> RVQKEGVLRVITRNSPATYFQDRNGETGFEYELAKRFAERLGVELKIETADNLDDLY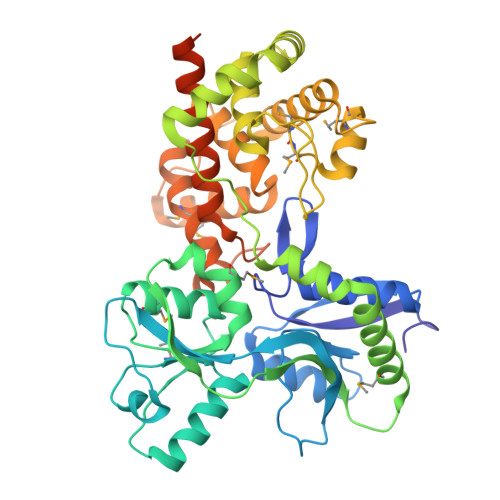AQLSREGGPALAAAGLTPGREDDASVRYSHTYLDVTPQIIYRNGQQRPTRPEDLVGKRIMVLKGSSHAEQLAELKKQYPELKYEESDAVEVVDLLRMVDVGDIDLTLVDSNELAMNQVYFPNVRVAFDFGEARGLAWALPGGDDDSLMNEVNAFLDQAKKEGLLQRLKDRYYGHVDVLGYVGAYTFTQHLQQRLPRYESHFKQSGKQKDTDWRLLAAIGYQESLWQPGATSKTGVRGLMMLTNRTAQAMGVSNRLDPKQSIQGGSKYFVQIRSELPESIKEPDRSWFALAAYNIGGAHLEDARKMAEKEGLNPNKWLDVKKMLPRLAQKQWYAKTRYGYARGGETVHFVQNVRRYYDILTWVTQPQMEGSQIAESGLHLPGVNKTRPEEDSGDEKL>[4x]MQDTIFLKGMRF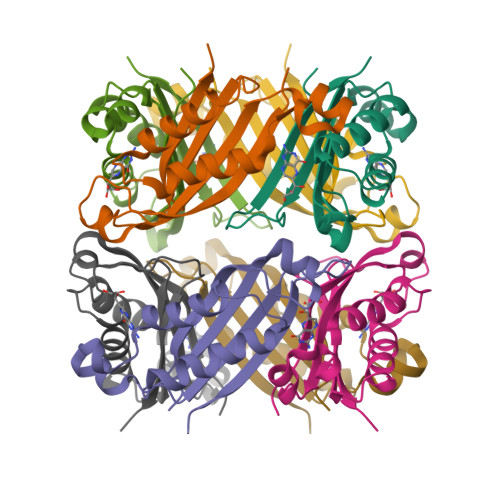YGYHGALSAENEIGQIFKVDVTLKVDLSEAGRTDNVIDTVHYGEVFEEVKSIMEGKAVNLLEHLAERIANRINSQYNRVMETKVRITKENPPIPGHYDGVGIEIVRENK> MVRNNNRRRQRTQRIVTTTTQTAPVPQQNVPKQPRRRRNRARRNRRQGRAMNMGALTRLSQPGLAFLKCA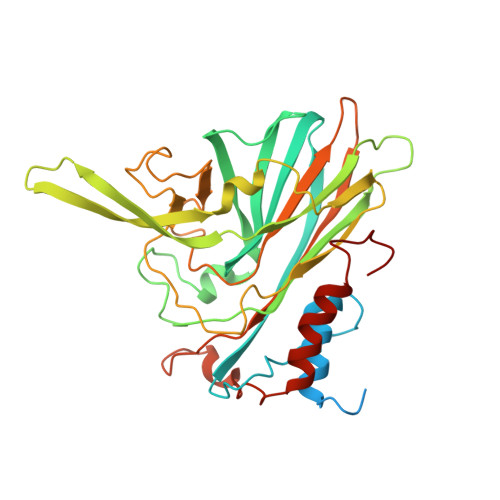FAPPDFNTDPGKGIPDRFEGKVVTRKDVLNQSINFTANRDTFILIAPTPGVAYWVADVPAGTFPISTTTFNAVNFPGFNSMFGNAAASRSDQVSSFRYASMNVGIYPTSNLMQFAGSITVWKCPVKLSNVQFPVATTPATSALVHTLVGLDGVLAVGPDNFSESFIKGVFSQSVCNEPDFEFSDILEGIQTLPPANVTVATSGQPFNLAAGAEAVSGIVGWGNMDTIVIRVSAPTGAVNSAILKTWACLEYRPNPNAMLYQFGHDSPPCDEVALQEYRTVARSLPVAVIAAQN> MKWYYKTITFLPELCNNESLAAKCLRVLHGFNYQYETRNIGVSFPLWCDATVGKKISFVSKNKIELDLLLKQHYFVQMEQLQYFHIS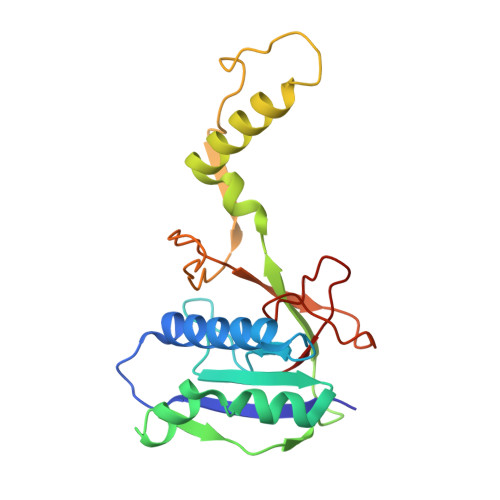NTVLVPEDCTYVSFRRCQSIDKLTAAGLARKIRRLEKRALSRGEQFDPSSFAQKEHTAIAHYHSLGESSKQTNRNFRLNIRMLSEQPREGNSIFSSYGLSNSENSFQPVPLI>MTIAKDANTFFGAESVQDPYPLYERMRAAGSVHRIANSDFYAVCGWDAVNEAIGRPEDFSSNLTATMTYTAEGTAKPFEMDPLGGPTHVLATADDPAHAVHRKLVLRHLAAKRIRV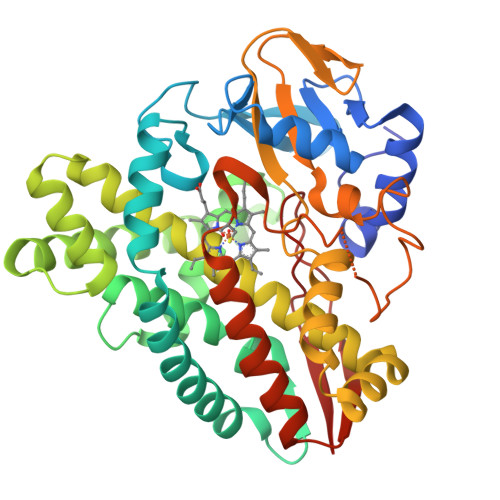MEQFTVQAADRLWVDGMQDGCIEWMGAMANRLPMMVVAELIGLPDPDIAQLVKWGYAATQLLEGLVENDQLVAAGVALMELSGYIFEQFDRAAADPRDNLLGELATACASGELDTLTAQVMMVTLFAAGGESTAALLGSAVWILATRPDIQQQVRANPELLGAFIEETLRYEPPFRGHYRHVRNATTLDGTELPADSHLLLLWGAANRDPAQFEAPGEFRLDRAGGKGHISFGKGAHFCVGAALARLEARIVLRLLLDRTSVIEAADVGGWLPSILVRRIERLELAVQ[2x]> LNTNQSVSARNQNARVRTRRAVAANDTEAPQVKSGDYVVYRGESFEYYAEITDNSGQVNRVVIRNVEGGANSTYLSPN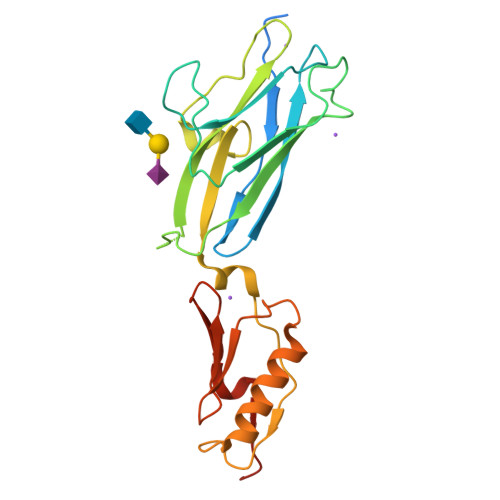WVKYSTENLGRPGNATVQNPLRTRIFGEVPLNEIVNEKSYYTRYIVAWDPSGNATQMVDNANRNGLERFVLTVKSQNEKYDPAESSVTYVNNLSNLSTSEREAVAAAVRAANPNIPPTAKITVSQNGTVTITYPDKSTDTIPANRVVKDLQISKSN> VAFIGITTGLLSLATVTGNLLVLISFKVNTELKTVNNYFLLSLACADLIIGTFSMNLYTTYLLMGHWALGTLACDLWLALDYVASNASVMNLLLISFDRYFSVTRPLSYRAKRTPRRAALMIGLAWLVSFVLWAPAILFWQYLVGERTVLAGQCYIQFLSQPIITFGTAMAAFYLPVTVMCTLYWRIYRETKRAGERLAKLLEKFEALPLEDIVAALKALLATNRPEIQLAVKTIVENFP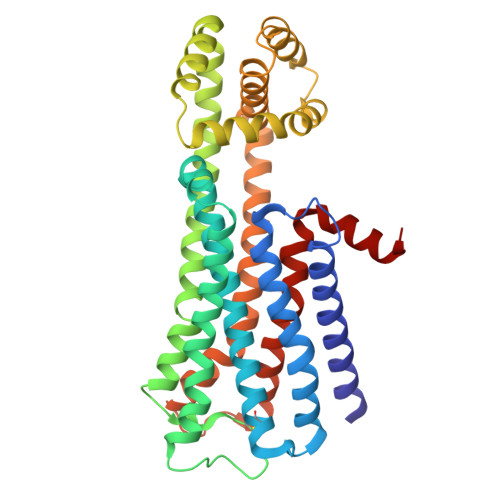EIKKEAEKLTPEQKAKLAALEAQLADLPEELRKVLLSMYLTGLLYGGSEENRKRAIEKAARTLSAILLAFILTWTPYNIMVLVSTFCKDCVPETLWELGYWLCYVNSTINPMCYALCNKAFRDTFRLLLLCR> MIKFLDLHKINQRFKSEIDLAIREVLESGWYLLGEKNKAFEENFAKYCETKFSVGCANGLDALHLAIRAYDFPKDSEIIVPANTYIASILAISNCGLKPILVEPNLETYNIDADLIEAKITEKTKAIVVVHLYGQAVEMEKIWELAKKYNLKIIEDCAQAHGAIYQGKKVGNLGDIGCFSFYPGKNLGALGDGGCITTNDEEMATKIRAIANYGSLIKYENIYKGLNSRLDEIQAAILDLKLQFLDADNQQRREIAKIYRENIKNEKIILPKPYEEESHVWHLFVIRT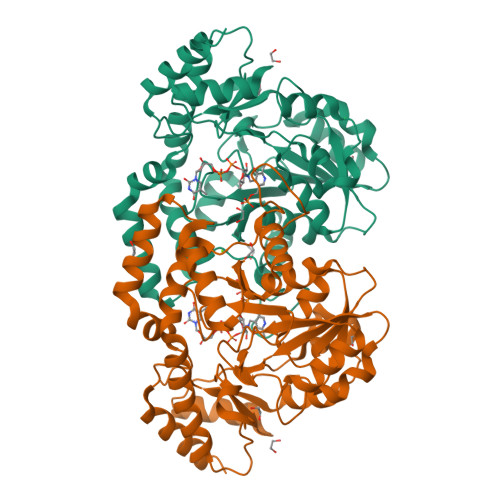KDRDKLQEYLKIKGIQTLIHYPIPPHKQNAYKEWNNLSFPITEKIHKEVLSLPISPVMNKEEAFYIAQILNEFLEHHHHHH> SSRGLLWDLLT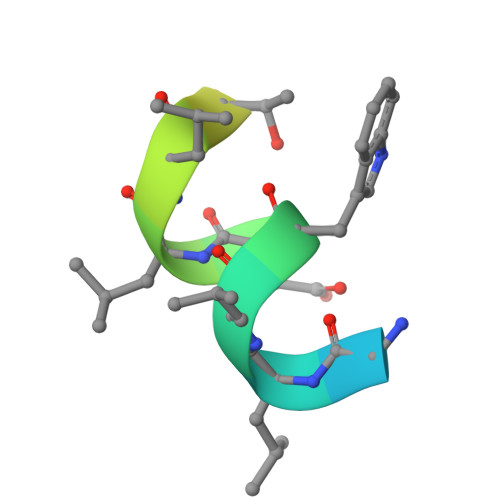KDSRSGSGK> IEIPMDPSIQNELTQPPTITKQSAKDHIVDPRDNILIECEAKGNPAPSFHWTRNSRFFNIAKDPRVSMRRRSGTLVIDFRSGGRPEEYEGEYQCFARNKFGTALSNRIRLQVSKSPLWPKENLDPVVVQEGAPLTLQCNPPPGLPSPVIFWMSSSMEPITQDKRVSQGHNGDLYFSNVMLQ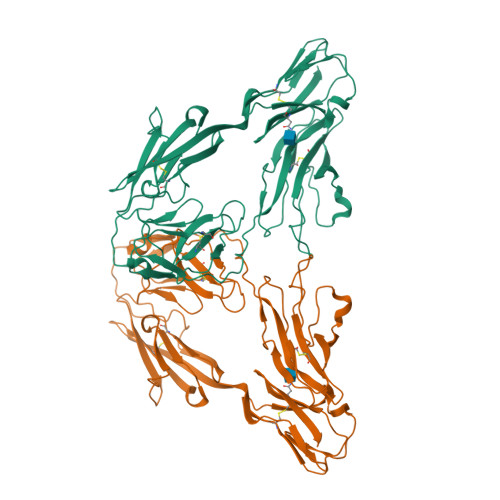DMQTDYSCNARFHFTHTIQQKNPFTLKVLTTRGVAERTPSFMYPQGTASSQMVLRGMDLLLECIASGVPTPDIAWYKKGGDLPSDKAKFENFNKALRITNVSEEDSGEYFCLASNKMGSIRHTISVRVKAAPYWLDEPKNLILAPGEDGRLVCRANGNPKPTVQWMVNGEPLQSAPPNPNREVAGDTIIFRDTQISSRAVYQCNTSNEHGYLLANAFVSVLDV> DGLSLSAGFDWTASILDQAQEEEESDQDQEDFTENKKHKHKRRKENVVQDKTIDINTRAPESVADFERLLIGNPNSSVVWMNYMAFQLQLSEIEKARELAERALKTINFREEAEKLNIWIAMLNLENTFGTEETLEEVFSRACQYMDSYTIHTKLLGIYEISEKFDKAAELFKATAKKFGGEKVSIWVSWGDFLISHNEEQ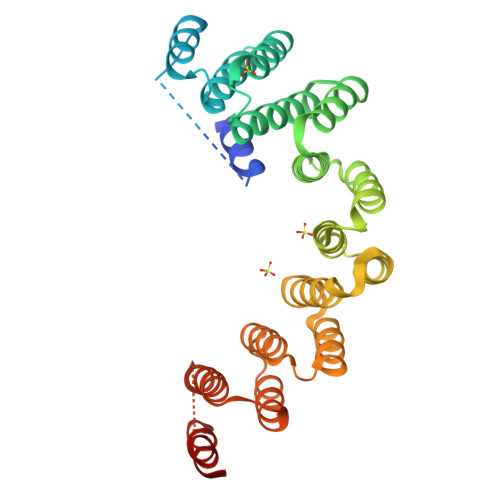EARTILGNALKALPKRNHIEVVRKFAQLEFAKGDPERGRSLFEGLVADAPKRIDLWNVYVDQEVKAKDKKKVEDLFERIITKKITRKQAKFFFNKWLQFEESEGDEKTIEYVKAKATEYVASHESQKADE> MTALGVEHDQHPACGGGSLTRHLQLIRLPGGGLSMLRFFCASLLLTG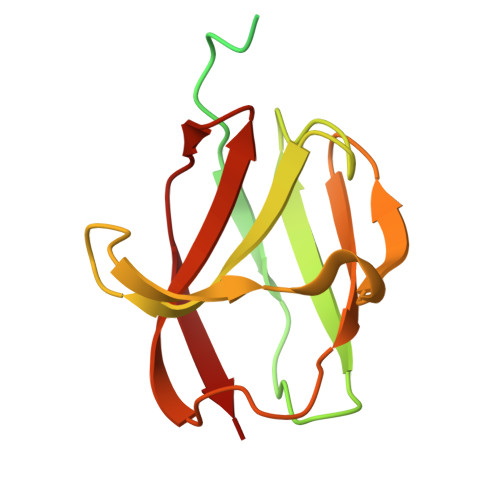LLASCTPRVTTVAGVTVTPVLIKVSEGAAPGDTLTIQGRYLGNAQTARVIIGADENGQGGTAFPASAVQSWSDTEIVLKVPEGMPAGGSWLFVEVGGKRSTGLRVSVR> SGVDDDMACHKIPVEADFLYAYSTAPGYYSWRNS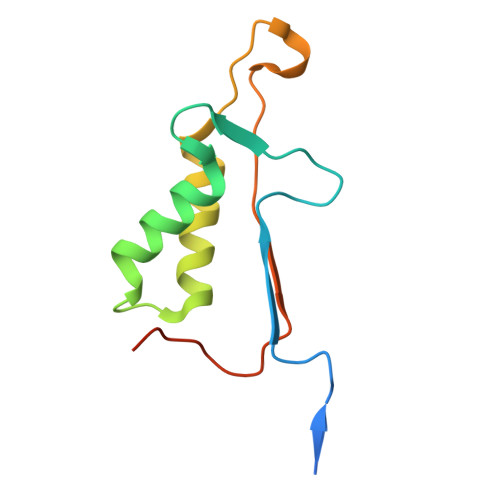KDGSWFIQSLCAMLKQYADKLEFMHILTRVNRKVATEFESFSFDATFHAKKQIPCIVSMLTKELYFYHHHHHHH> T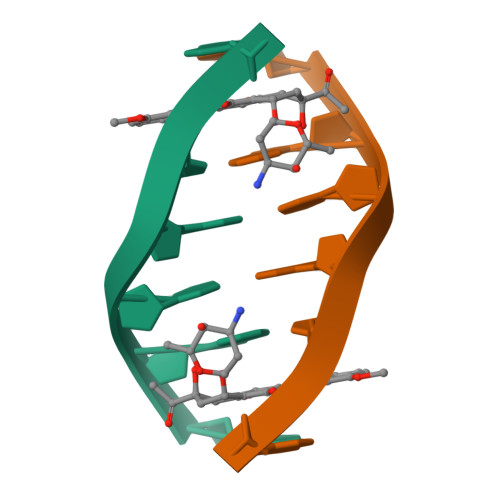GTACA N~2~,N~2~-DIMETHYL-N~1~-(6-OXO-5,6-DIHYDROPHENANTHRIDIN-2-YL)GLYCINAMIDE | C17 H17 N3 O2 | 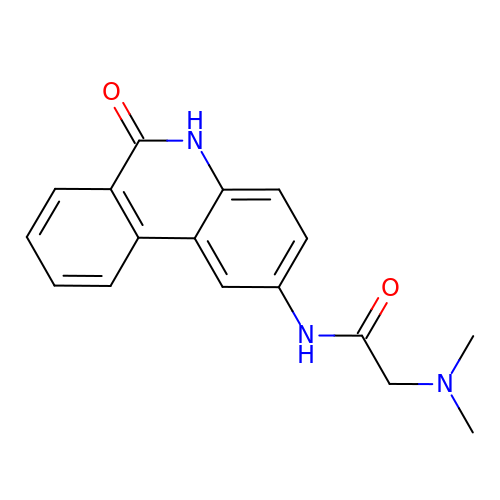UYJZZVDLGDDTCL-UHFFFAOYSA-N>[6x]MAHHHH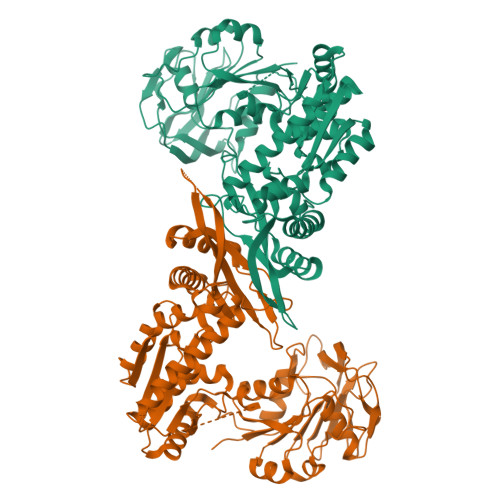HHMTQDKILILDFGSQVTRLIARRVREAHVYCELHSFDMPLDEIKAFNPKGIILSGGPNSVYESDYQADTGIFDLGIPVLGICYGMQFMAHHLGGEVQPGNQREFGYAQVKTIDSGLTRGIQDDAPNTLDVWMSHGDKVSKLPDGFAVIGDTPSCPIAMMENTEKQFYGIQFHPEVTHTKQGRALLNRFVLDICGAQPGWTMPNYIEEAVAKIREQVGSDEVILGLSGGVDSSVAAALIHRAIGDQLTCVFVDHGLLRLNEGKMVMDMFARNLGVKVIHVDAEGQFMAKLAGVTDPEKKRKIIGAEFIEVFDAEEKKLTNAKWLAQGTIYPDVIESAGAKTKKAHAIKSHHNVGGLPENMKLKLLEPLRDLFKDEVRELGVALGLPREMVYRHPFPGPGLGVRILGEVKKEYADLLRQADDIFIQELRNTTDENGTSWYDLTSQAFAVFLPVKSVGVMGDGRTYDYVVALRAVITSDFMTAHWAELPYSLLGRVSNRIINEVKGINRVVYDVSGKPPATIEWE> MENTENSVDSKSIKNLEPKIIHGSESMDSGISLDNSYKMDYPEMGLCIIINNKNFHKSTGMTSRSGTDVDAANLRETFRNLKYEVRNKNDLTREEIVELMRDVSKEDHSKRSSFVCVLLSHGEEGIIFGTNGPVDLKKITNFFRGDRCRSLTGKPKLFIIQACRGTELDCGIETDSGVDDDMACHKIPV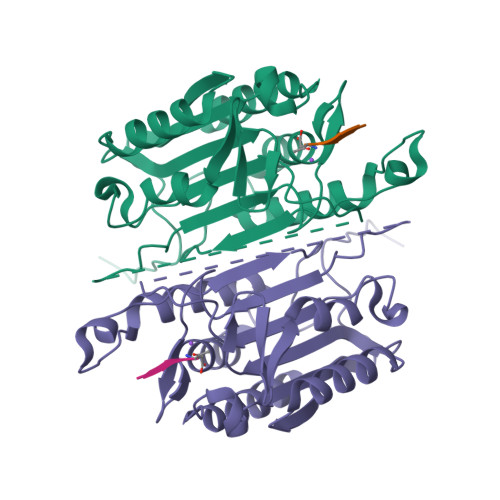EADFLYAYSTAPGYYSWRNSKDGSWFIQSLCAMLKQYADKLEFMHILTRVNRKVATEFESFSFDATFHAKKQIPCILSMLTKELYFYHL>MITQEMKDLINNQLAMVATVDAKGQPNIGPKRSMRLWDDKTFIYNENT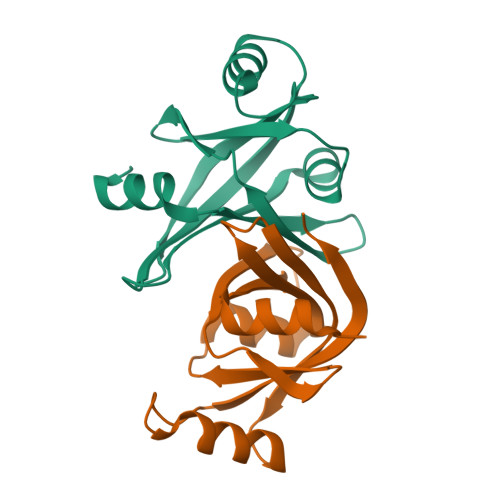DGQTRINIEDNGKIEIAFVDRERLLGYRFVGTAEIQTEGAYYEAAKKWAQGRMGVPKAVGIIHVERIFNLQSGANAGKEINSESN[4x]>ARKCSLTGKWTNNLGSIMTIRAVNSRGEFTGTYLTAVADNPGNITLSPLLGIQHKRASQPTFGFTVHWNFSESTTVFTGQCFIDRNGKEV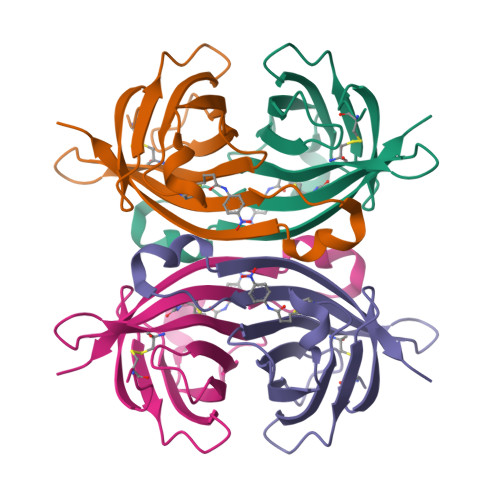LKTMWLLRSSVNDISYDWKATRVGYNNFTRLS[2x]>GGYMLGS[2x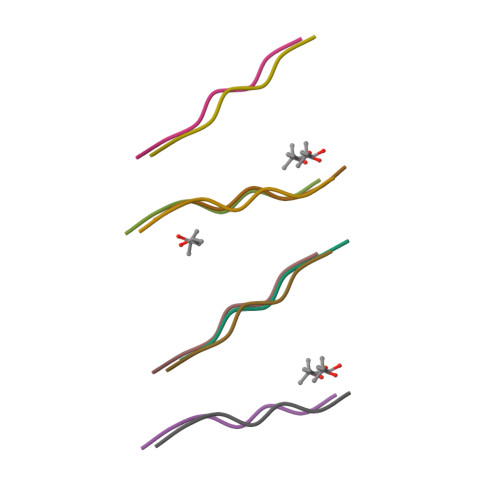]> MTVPDEPVG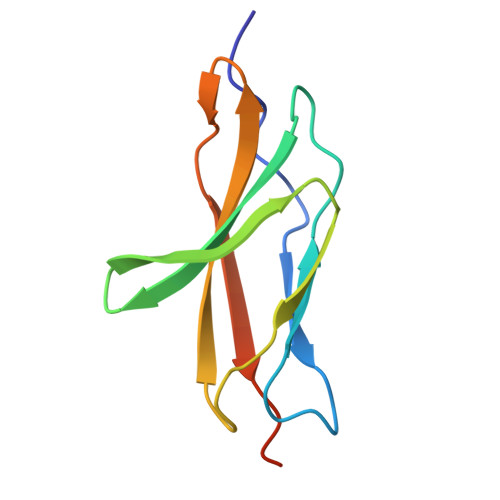FWVESIPGNDHTLRLRWSETKGAKYYEIYLVSDSTYKFIASTDKLEYYVTNLSPNTKYCFALRAVNELGPSNFVTASSTTDRGGHHHHHH>MGGEVEEPEPQMVLSPLTSAAIFLVVTIDSGGEDTVRDLLSDVASLERAVGFRAQPDGRLSCVTGIGSEAWDRLFSGARPAGLHPFRELDGPVHRAVATPGDLLFHIRASRLDLCFALATEIMGRLRGAVTPQDEVHGFKYFDERDMLGFVDGTENPTGAAARRAVLVGAEDPAFAGGSYAVVQKYLHDIDAWEGLSVEAQERVIGRRKMTDVELSDDVKPADSHVALTSVTGPDGSDLEILRDAMPFGSVGREEFGTYFIGYARTPEVTETMLERMFLGTASAPHD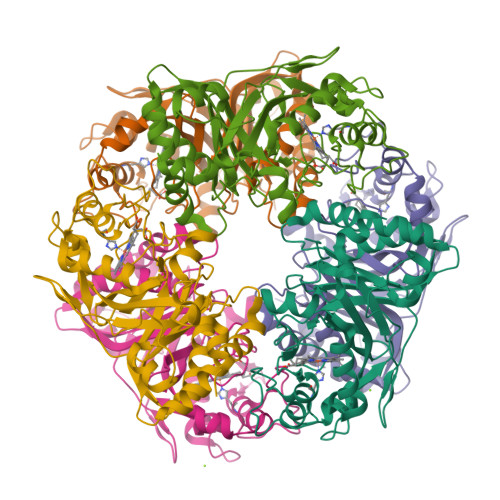RILDFSTAVTGSLFFTPAADFLEDLSARP[6x]> XD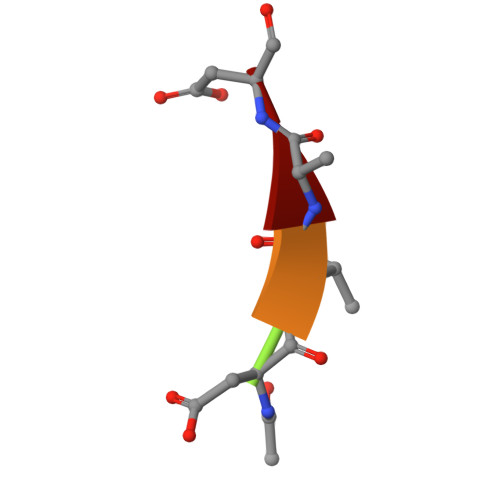VAD> MRGSHHHHHHGSSKKTTTVGVIIPDISSIFYSELARGIEDIATMYKYNIILSNSDQNMEKELHLLNTMLGKQVDGIVFMGGNITDEHVAEFKRSPVPIVLAASVEEQEETPSVAIDYEQAIYDAVKLLVDKGHTDIAFVSGPMAEPINRSKKLQGYKRALEEANLPFNEQFVAEGDYTYDSGLEALQHLMSLDKKPTAILSATDEMA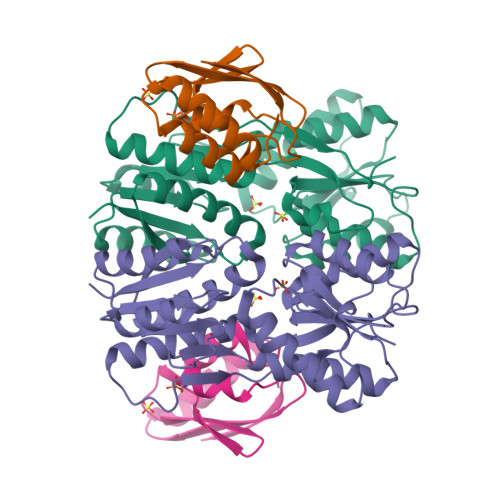LGIIHAAQDQGLSIPEDLDIIGFDNTRLSLMVRPQLSTVVQPTYDIGAVAMRLLTKLMNKEPVEEHIVELPHRIELRKSTKS;> MAQKTFKVTADSGIHARPATVLVQTASKYDADVNLEYNGKTVNLKSIMGVMSLGIAKGAEITISASGADENDALNALEETMKSEGLGE>GVWRQYASRALQELGAGKRAIHDVADLTRGSLRIAVTPTFTSYFIGPLMADFYARYPSITLQLQEMSQEKIEDMLCRDELDVGIAFAPVHSPELEAIPLLTESLALVVAQHHPLAVHEQVALSRLHDEKLVLLSAEFATREQIDHYCEKAGLHPQVVIEANSISAVLELIRRTSLSTLLPAAIATQHDGLKAISLAPPLLERTAVLLRRKNSWQTAAAKAFL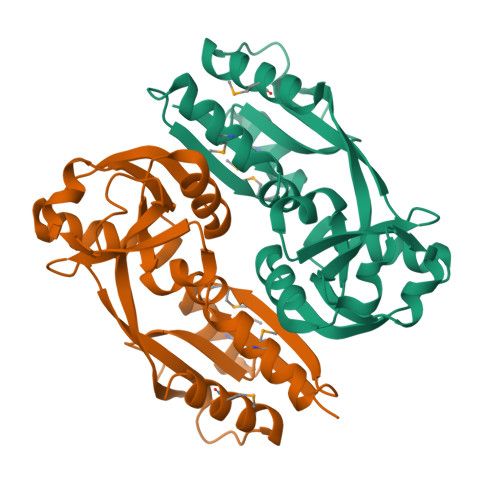HMALDKCAVVGGNESR[2x]>[3x]RGSHHHHHHGSFTPSGTTGTTKLTVTEKCQVRVGDLTVAKTRGQLTDAAPIGPVTVQALGCDARQVALKADTDNFEQGKFFLISDNNRDKLYVNIRPTDNSAWTTDNGVFYKNDVGSWGGIIGIYVDGQQTNTPPGNYTLTLTGGYWAK

Dr adhesins are expressed on the surface of uropathogenic and diffusely adherent strains of Escherichia coli. The major adhesin subunit (DraE/AfaE) of these organelles mediates attachment of the bacterium to the surface of the host cell and possibly intracellular invasion through its recognition of the complement regulator decay-accelerating factor (DAF) and/or members of the carcinoembryonic antigen (CEA) family. The adhesin subunit of the Dr haemagglutinin, a Dr-family member, additionally binds type IV collagen and is inhibited in all its receptor interactions by the antibiotic chloram­phenicol (CLM). In this study, previous structural work is built upon by reporting the X-ray structures of DraE bound to two chloramphenicol derivatives: chloramphenicol succinate (CLS) and bromamphenicol (BRM).

A unique CLS cocrystal in space group C2 was obtained at a small-molecule concentration of 10 mM and could not be reproduced. All the cocrystals described in this work belong to the P3 form (with the exception of a single irreproducible C2 DraE–CLS crystal that grew in 10 mM CLS); both C2 and P3 crystals contain DraE trimers, as did the apo P212121 crystals (and the related AfaE-III cubic and trigonal crystals). Ordering of the whole ligand in the P3 forms is helped by crystal contacts from a neighbouring protein molecule (Gln47 and Leu49) to the ligand atoms C7 and C8 (in the phenyl ring) and one of the O atoms on the nitro moiety (the atom labelled O9B); this crystal contact is missing in the C2 form and the ‘head group’ of CLS adopted a number of conformations that were not traceable. In addition, the disordered nitrobenzene group in the DraE–CLS structure in space group C2 implies that the interaction with DraE is focused on the burial of the chlorines rather than the benzene ring. This raises the possibility that the nitrobenzene group is not required for DAF inhibition. Overall, the CLS–DraE complex structures imply that (i) substitutions at the primary hydroxyl do not significantly affect the mode of CLM binding and (ii) the nitrobenzene group is not required to bind DraE.> DTATLGELAEAKGRYFGSATDNPELPDTQYTQILGSEFSQITVGNTMKWQYTEPSRGRFDYTAAEE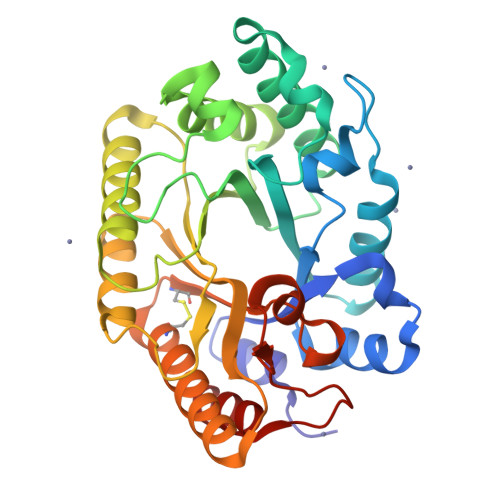IVDLAESNGQSVRGHTLVWHNQLPSWVDDVPAGELLGVMRDHITHEVDHFKGRLIHWDVVNEAFEEDGSRRQSVFQQKIGDSYIAEAFKAARAADPDVKLYYNDYNIEGIGPKSDAVYEMVKSFKAQGIPIDGVGMQAHLIAGQVPASLQENIRRFADLGVDVALTELDIRMTLPRTAAKDAQQATDYGAVVEACLVVSRCVGITVWDYTDKYSWVPSVFPGQGAALPWDEDFAKKPAYHAIAAALN> MGSSHHHHHHSQDPNSMPDNTIQWDKDADGIVTLTMDDPSGSTNVMNEAYIESMGKAVDRLVAEKDSITGVVVASAKKTFFAGGDVKTMIQARPEDAGDVFNTVETIKRQLRTLETLGKPVVAAINGAALGGGLEIALACHHRIAADVKGSQLGLPEVTLGLLPGGGGVTRTVRMFGIQNAFVSVLAQGTRFKPAKAKEIGLVDELVATVEELVPAAKAWIKEELKANPDGAGVQPWDKKGYKMPGGTPSSPGLAAILPSFPSNLRKQLKGAPMPAPRAILAAAVEGAQVDFDTASRIESRYFASLVTGQVAKNMMQAFFFDLQAINAGGSRPEGIGKTPIKRIGVLGAGMMGAGIAYVSAKAGYEVVLKDVSLEAAAKGKGYSEKLEAKALERGRTTQERSDALLARITPTADAADFKGVDFVIEAVFENQELKHKVFGEIEDIVEPNAILGSNTSTLPITGLATGVK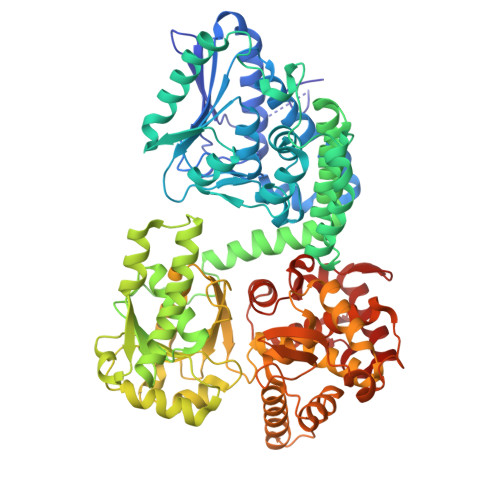RQEDFIGIHFFSPVDKMPLVEIIKGEKTSDEALARVFDYTLAIGKTPIVVNDSRGFFTSRVIGTFVNEALAMLGEGVEPASIEQAGSQAGYPAPPLQLSDELNLELMHKIAVATRKGVEDAGGTYQPHPAEAVVEKMIELGRSGRLKGAGFYEYADGKRSGLWPGLRETFKSGSSQPPLQDMIDRMLFAEALETQKCLDEGVLTSTADANIGSIMGIGFPPWTGGSAQFIVGYSGPAGTGKAAFVARARELAAAYGDRFLPPESLLS>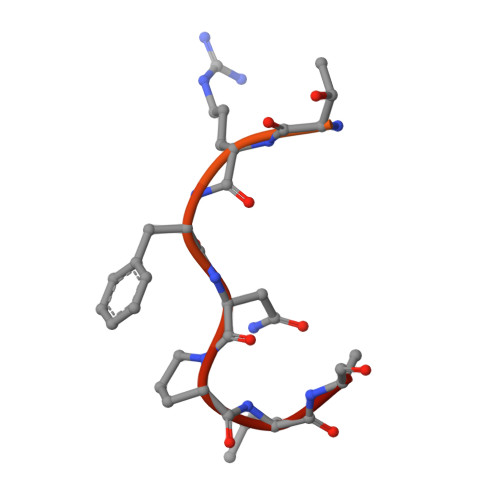 RFTQRGGGAVGKNRRGGRGGNRGGRNNNSTRFNPLAKA>[4x]TIRSGDDYIESLRGRDLKVYLFGELVKEPVDHPMIRPSINAVAETYDLALREEALASADSSITGLKVNRFLHIAESAEDLVLQNKMQRKLGQNTG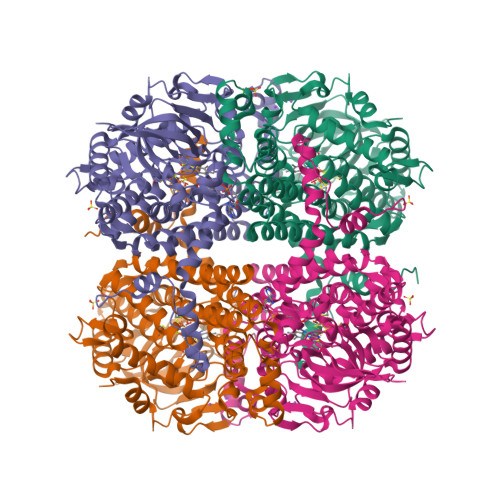TCFQRCVGMDAMNSLHSTTFEIDEKHGTDYHKRFLEFVKMVQQENLVIGGAMTDPKGDRSKGPSEQDDPDLFTRIVDTDEKGVYVSGAKAHQTGCINSHWIILMPTIRLTESDKDWAIVGAIPADAKGVTYIYGRQSCDTRSMEEGDIDDGNAKFGGQEALIILDRVFIPWDKVFMHGEYEFASMLVERFTCYHRRSYVCKTGLGDVLIGAAATIADYNGVPKVSHIKDKIIEMTHLNETIFAAGIASSHQGQKMKSGVYLNDDMLAQVCKHNVTRFPYEISRLAQDIAGGLVVTLPSEKDFRHPEAGPLLKKYLAGRKGVDVENRMRILRLIENMTLGRNAVGYLTESMHGAGSPQAQRIQIQRQMQVGYKKNLAKNLAGITNDVEEPKESSEYFKRVFKTKDSVL>[2x]MKSYFVTMGFNETFLLRLLNETSAQKEDSLVIVVPSPIVSGTRAAIESLRAQ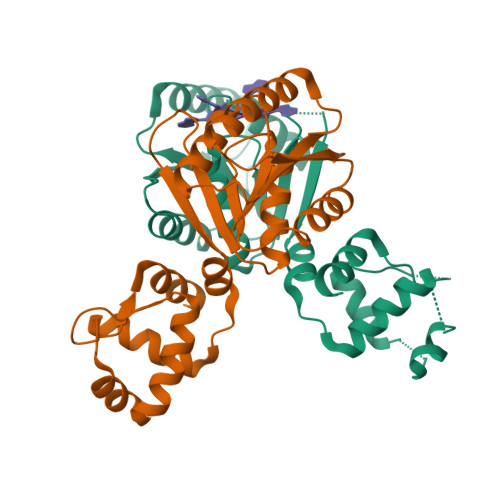ISRLNYPPPRIYEIEITDFNLALSKILDIILTLPEPIISDLTMGMRMINTLILLGIIVSRKRFTVYVRDEGGGSRVISFNDNTIRALMRDYSREEMKLLNVLYETKGTGITELAKMLDKSEKTLINKIAELKKFGILTQKGKDRKVELNELGLNVIKLNK ADENOSINE-5'-[TRIHYDROGEN DIPHOSPHATE] P'-3'-ESTER WITH 2'-DEOXYURIDINE 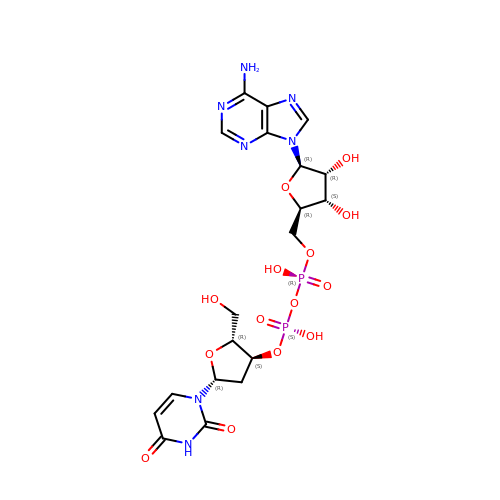| C19 H25 N7 O14 P2 | NGHFJGUDQJTSRY-LNAOLWRRSA-N>MMCLKLNLLDHVFANPFMNAAGVLCSTEEDLRCMTASSSGALVSKSCTSAPRDGNPEPRYMAFPLGSINSMGLPNLGFDFYLKYASDLHDYSKKPLFLSISGLSVEENVAMVRRLAPVAQEKGVLLELNLSCPNVPGKPQVAYDFEAMRTYLQQVSLAYGLPFGVKMPPYFDIAHFDTAAAVLNEFPLVKFVTCVNSVGNGLVIDAESESVVIKPKQGFGGLGGKYILPTALANVNAFYRRC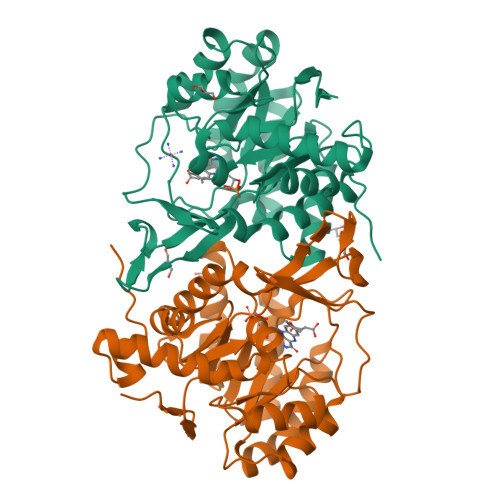PDKLVFGCGGVYSGEDAFLHILAGASMVQVGTALQEEGPGIFTRLEDELLEIMARKGYRTLEEFRGRVKTIE[2x]> GPDSMSEGFSSSSIQELYQSLKEITNNADVELFEDRITKLDFESTDEPKHANDIIKDRFLRPSNALPWSLLDMVQDVPHTSSPEDCSGKLDYKELLKVPDPINRTSYQFKRTGLEGKISGYKEEVDLKEVANANASNSLSITRSINHNQNSVRGSTAQLPFTPGGIPMKSVKTDSEQNGSSTMANATKLLHKDGQGLFDIPEGMNRGIKPMDXXXXXXXXXXXXXXXXXXXXXXXXXXXXXXXXXXXXXXXXXXXXXXXXXXXXXXXXXXXXXXXXXXXXXXXXXXXXXXXXXXXXXXXXXXXXEWAHVVDLNHKIENFDELIPNPARSWPFELDTFQKEAVYHLEQGDSVFVAAHTSAGKTVVAEYAIAMAHRNMTKTIYTSPIKALSNQKFRDFKETFDDVNIGLITGDVQINPDANCLIMTTEILRSMLYRGADLIRDVEFVIFDEVHYVNDQDRGVVWEEVIIMLPQHVKFILLSATVPNTYEFANWIGRTKQKNIYVISTPKRPVPLEINIWAKKELIPVINQNSEFLEANFRKHKEILNGESAKGAPSKTDNGRGGSTARGGRGGSNTRDGRGGRGNSTRGGANRGGSRGAGAIGSNKRKFFTQ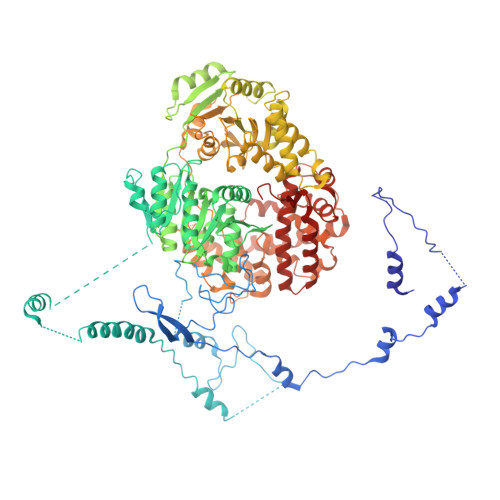DGPSKKTWPEIVNYLRKRELLPMVVFVFSKKRCEEYADWLEGINFCNNKEKSQIHMFIEKSITRLKKEDRDLPQILKTRSLLERGIAVHHGGLLPIVKELIEILFSKGFIKVLFATETFAMGLNLPTRTVIFSSIRKHDGNGLRELTPGEFTQMAGRAGRRGLDSTGTVIVMAYNSPLSIATFKEVTMGVPTRLQSQFRLTYNMILNLLRIEALRVEEMIKYSFSENAGSRGLSLLPDYEKRLAVLKDTEFIDQNHNVLLKGRVACEINSGYELVLTELILDNFLGSFEPEEIVALLSVFVYEGKTREEEPPIVTPRLAKGKQRIEEIYKKMLCVFNTHQIPLTQDEAEFLDRKRFAMMNVVYEWARGLSFKEIMEMSPEAEGTVVRVITWLDEICREVKTASIIIGNSTLHMKMSRAQELIKRDIVFAASLYL> GAMVSCPICMDGYSEIVQNGRLIVSTECGHVFCSQCLRDSLKNANTCPTCRKKIN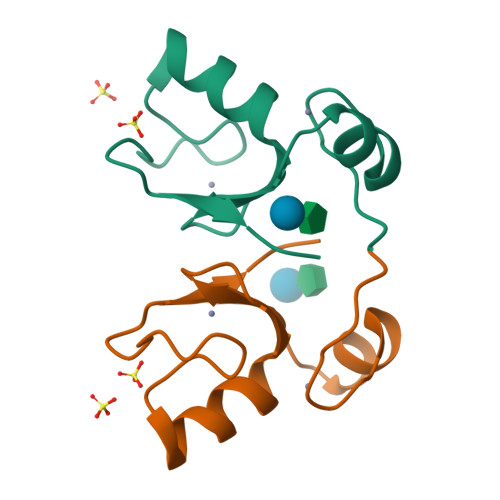HKRYHPIYI> PLPEVQCFVFNIEYMNCTWNSSSEPQATNLTLHYRYKVSDNNTFQECSHYLFSKEITS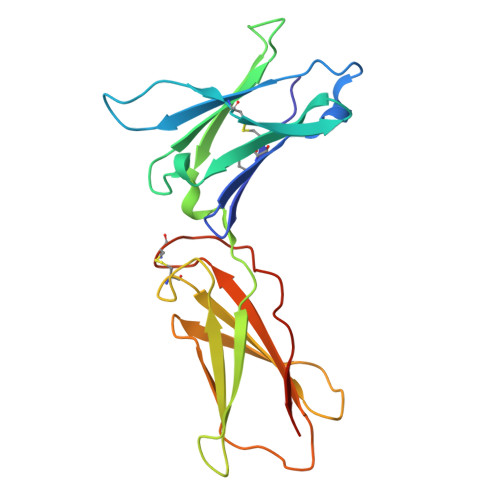GCQIQKEDIQLYQTFVVQLQDPQKPQRRAVQKLNLQNLVIPRAPENLTLSNLSESQLELRWKSRHIKERCLQYLVQYRSNRDRSWTELIVNHEPRFSLPSVDELKRYTFRVRSRYNPICGSSQQWSKWSQPVHWGSHTVEE>[12x]MGSSHHHHHHSSGRENLYFQGMPHLVIEATANLRLETSPGELLEQANAALFASGQFGEADIKSRFVTLEAYRQGTAAVERAYLHA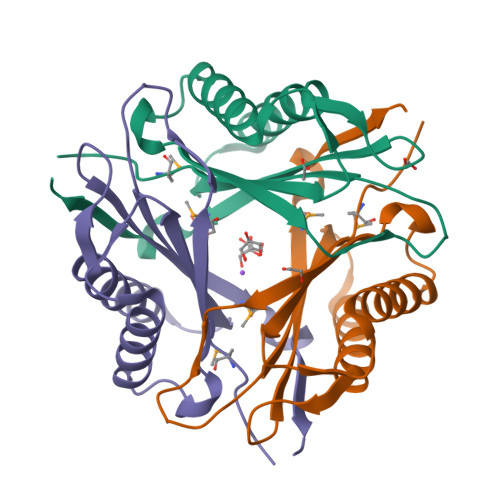CLSILDGRDAATRQALGESLCEVLAGAVAGGGEEGVQVSVEVREMERASYAKRVVARQRGS> IVGGYTCGANTVPYQVSLNSGYHFCGGSLINSQWVVSAAHCYKSGIQVRLGEDNINVVEGNEQFISASKSIVHPSYNSNTLNNDIMLIKLKSAASLNSRVASISLPTSCASAGTQCLISGWGNTKSSGTSYPDVLKCLKAPI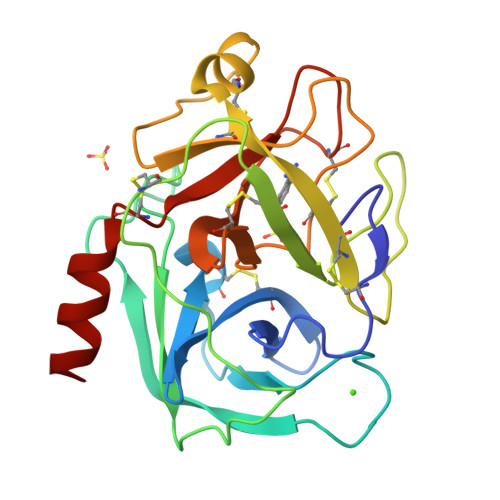LSDSSCKSASSFIITSNMFCAGYLEGGKDSCQGDSGGPVVCSGKLQGIVSWGEGCAQKNKPGVYTKVCNYVSWIKQTIASN> MESGIDLQGQFISALQSLGLSHDLAKLLWLPLPMLMMLIVATVGVLVAVWLERKISAAVQQRIGPEYIGPLGILAPLADGLKLIFKEDVLPANSDRWLFTLGPAVVVIPVFLSYIIVPFGQNLLISNLAMGVFLWIALSSIAPIGLLMAGYASNNKYSLLGGLRAAAQSISYEIPLALAVLAVAMMSNGLGTVEIVEQQSQYGILSWNVWRQPIGFLVFWIAALAECERLPFDLPEAEEELVAGYQTEYAGMKFALFYLGAYVNLVLSALLVSVLYFGGWSFPIPLETIANLLGVSETNPFLQIAFAVLGITMTLIKAYFFVFLAILLRWTVPRVRIDQLLDLGWKFLLPVGLVNLLLTAGLKLAFPVAFGG;> MDLVTLAGQLNAGTILPETILIVTLLVVLLADLIQGRQADRWTPYFAIVGLGGAIATMIPLWTQPATISFFGSFISDHLSLFFRGLIALSALGTILMSIRYVEQTGSSLGEFMTILLTATVGGMFIAGAQELVFIFVALETLSIASYLLTGYTKRDSRSNEAALKYLLIGAASSAIFLYGSSLLYGLSGGHTQLPAIAQALSSESLGLVVALVFVIAGISFKISAVPFHQWTPDVYEGAPTPVVAFLSVGSKAAGFALAIRFLTLAFPSVTDQWQLIFTVLAILSMILGNVVALAQTSMKRMLAYSSIGQAGFVMIGFVVGTEAGYASMLFYLLVYLFMNLGAFTCVILFSLRTGTDQISEYAGLYQKDPLLTLGLSLCLLSLGGIPPLAGFFGKIYLFWAGWQAGAYGLVLLGLLTSVISIYYYIRVVKMMVVKEPQEMSEAVRNYPEVSWSSFGLRPLQVGLVMTVIATSLAGILANPLFNLVNTAVWDVPQLANQPTVMEVAYQALSPAGKS;> MVAIPRLRDTATVFVLSGYEYFLGFLIICSLVPVLALAASALLRPKSGRMIRLTTYESGMEPIGGAWIQFNVRYYMFALVFVIFDVETVFLYPWAVAFHQLGLLAFIEALIFIAILVVALVYAWRKRALEWS;> MSTFPWLTTIILFPIVAALAIPFIPDPTGKGRPIRWYALAVGLIDFALIVYAFTNFYDLNTPGMQLWESYDWIPEIGLRWSVGADGLSMPLILLTGFITTLAILAAWPVTLKPRLFYFLMLAMYGGQIAVFAVQDMLVFFLAWELELIPVYLLLAIWGGHKRQYAATKFILYTAGSSLFILVAGLAMAFYGDTVSFDMQTLAAKDYALGFQLLVYAGFLVAYGVKLPIVPLHTWLPDAHGEATAPVHMLLAGILLKMGGYALIRMNVDMLPAAHAKFAPVLVILGVVNIIYAALTSYAQRNLKRKIAYSSISHIGFVLIGIASFTNLGMSGAVLQMVSHGLIGASLFFLVGATYDRTHTLILEEMGGVGQKMKKIFAMFTACSLASLALPGMSGFVAELMVFIGFATSDAYSLPFRVIVVFLAAVGVILTPIYLLSMLREIFYGPENKELVEHEALVDAEPREVFIIACLLVPIIGIGLYPKLLTQIYDATTGQVIARAREVLPTLAQQTEQPLGILPMVAPQLKANAQ;> MQLTYVLILAALLFCIGIYGLVTSRNAVRVLMSIELLLNAVNLNLIGFANYLDGQQIKGQVFAVFVITVAAAEAAVGLAIILAIYRNRDTVDMEKFNLLKW;> MEPLYQYAWLIPVLPLLGALIVGFGLIAFSETTSKLRRPSAIFIMALMAIAMGHSLTLFWSQVQGHLPYTQMIEWAAAGNLHIAMGYVIDPLAALMLVIVTTVAFLVMLYSDGYMAHDPGYVRFFAYLSLFGSSMLGLVVSPNLVQVYIFWELVGMCSYLLIGFWYDRKSAAEAAQKAFVTNRVGDFGLLLGMVGLFWATGTFDFAGMGDRLTELVNTGLLSPSLAAILAILVFLGPVAKSAQFPLHVWLPDAMEGPTPISALIHAATMVAAGVFLIARMFPVFEQLPQVMTTIAWTGAFTAFMGATIAITQNDIKKSLAYSTISQLGYMVMGMGVGAYSAGLFHLMTHAYFKAMLFLGSGSVIHSMEGVVGHNPDLAQDMRYMGGLRKYMPITGATFLVGCLAISGVPPFAGFWSKDEILGAVFHANPAMWLLTWLTAGLTAFYMFRMYFMTFEGKFRNVPPERQEHHDHHSHHAAVPHESPWTMTLPLVVLAIPSTLIGFVGTPFNNLFEVFIHAPGEEKVAEHAVDLTEFLILGGSSVGIGLMGITVAYLMYLKGTPSPQAIAKAIQPLYQFSLHKWYFDELYEAVFIKGCRRLARQVLEVDYN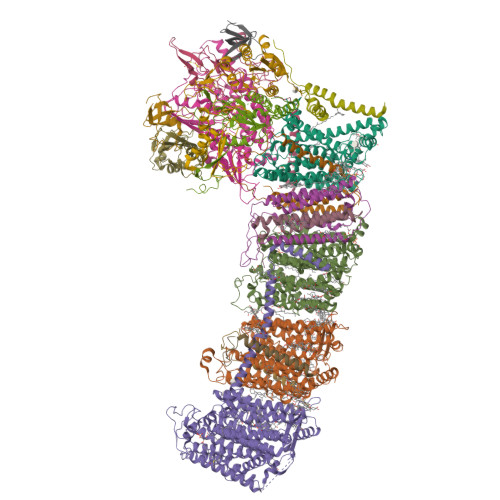VVDGVVNLTGFVTMVTGEGLKYLQNGRAQFYALIVLLAVLGFVIFSVQT;> MDLATLTQTITFFALAAAVIIAALGVVLLDNVVYSAFLLGGVFLSIAGLYILMNADFVSAAQILIYVGAVNVLILFAIMLVNKRETYTPVPGRWLRQGGAAVVSLGVFALLTKMILQTPWQLSSVPPTPDSITTIGQHFFSDFLLPFELASVLLLMALIGAVVLARRELVLEPEPILGEEVVPPLELPERPREPVALSEK;> MPKIETRTEPMVINMGPHHPSMHGVLRLMVTLDGEDVIDCEPVIGYLHRGMEKIAENRTNIMFIPYVSRWDYAAGMFNEAVTVNAPEKLAGIPVPKRASYIRVIMLELNRIANHLLWLGPFLADVGAQTPFFYIFREREYIYDLFEAATGMRFINNNYFRIGGVAADLTYGWVTKCRDFCDYFLPKVDEYERLITNNPIFVRRLQGVGKISREEAINWGLSGPMLRASGVKWDLRKVDHYECYDDFDWDVPVATEGDCLARYIVRIQEMRESVKIIRQALDGLPGGPYENLEAKRMLEGAKSEWNGFDYQYIGKKLSPTFKIPKGEHYVRVESGKGELGIYLIGDDNVFPWRWKIRPPDFNNLQVLPQLLKGMKVADIVAILGSIDVIMGSVDR;> MKFLNQITNYAKEAVQSAKYIGQGLSVTFDHMRRRPITVQYPYEKLIPSERFRGRIHFEFDKCIACEVCVRVCPINLPVVDWVFNKELKKKELKHYSIDFGVCIFCANCVEYCPTNCLSVTEEYELATYDRHELNYDSVAMGRIPYKVTQDPMVTPIREFAYLPAGVMSGHDLPAGAQRAGERPEAIANTAKSSEN;> MSDTPEAPIVEAGPVGRLLQSQNLSVESLGRDASGVEMIKVDRDRLLAVCQTLYADGFNYLRCQAAYDSGPGQDLVSTYHLIKLSDNADRPPEVRIKVFVPRDDPRVPSVYWIWKTADWQERESYDMFGIVYEGHPNLKRILMPEDWVGWPLRKDYITPDFYELQEAY;> MTNTTSPAILNPIARPEVPQELAENIILTSLNDVYDWARLSSLWPLMYGTACCFIEFAAMIGSRFDFDRFGLVPRNSPRQADLIITSGTITMKMAPALVRLYEQMPSPKYVIAMGACTITGGMFSSDSYSAVRGVDKLIPVDVYLPGCPPRPEAIMDAIVKLRKKIANEHINERGNLAQTHRLFTAKHKMKPVPPILTGQYLNAPSRQAPPPALAAAMGIAVPALGEAVSETTSVAE;> MAVSTELLVLGVYGALAGLYLLVVPAIVYAYLNARWYVASSFERAFMYFLVTFFFPGLLLLAPFINFRPQPRSLNS;> MLLKSTTRHVHIYAGHVVDGEVHPDTETLTLNVDPDNELEWNEAALAKVEAKFRELVANAAGEDLTEYNLRRIGSDLEHFIRSLLMQGEIGYNLNSRVRNYSLGIPRVNHS;> MGLLAGYQFVKDLESAGALALFVPPEGGFEGRYQRRLRSKGYTTLPMSAPGLGDLAAYLTQEHGIRPAHTGKEDIRVYFQPPLVTYHLENLPPNAKGLVLWLIDGKRLSKQEFAYLAQLTQTLPKFKVVVEVGGDRVVRWEPLADWVAAA;> MAIKKGDLVKVVAEKLANSLEALASDHRYPPYLFEGRGEVVDIRGDYAQIKFPVPTPTVWLRLDQLEVAQ;> MDAVISVKPILLAMTPVFILLCLFFGTRNGFYDTDQYHGNGSAH;> MATDFNRGIMKFDGADSPAMIAISAVLILGFIAGLIWWALHTAYA;> MIRPIADTYPLLPLSKAQMGQRQEIINSHKRLWDKTMATDLIMTILPGMTVKVTNPNDTYYQFQGIVQRITDGKVAVLFEGGNWDKLVTFQASELEPVVVTPKEKAKAKK> MCELYLDSPNLGELEKEYILKAIDSNFVSTVGPFVPEFEEKFAKYLRVTSCVAVQSGTAAIHAALYELGIKEGDEIIVPAITFVATVNPIVYCGATPVFVDIDKDTWDIDPKEIEKSITSKTKAIIPVHLYGNPCDMDEIMKIAEKYGLYVIEDATESLGAEYKGRMTGTIGHIGCFSFNGNKIITTG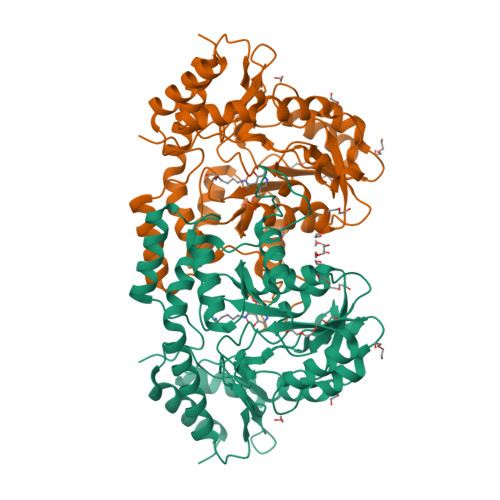GGGMISTNNEKWASHIKFLVNQARDASQGYFHPEIGFNYRMTNLEAALGLAQLERLPEFLKKKRMYFEAYKKIFGGIDEIALQKEYEGAISSAWLPSIKIDRKKIKMTIPEIQDKLKEKGIPTRRIFNPIVDFPPYVKYKNGNYHNSYEIFENGLSLPASTLNTLENIEYAAKTLLNILGIKKEVIL> FACKTANGTAIPIGGGSANVYVNLAPVVNVGQNLVVDLSTQIFCHNDYPETITDYVTL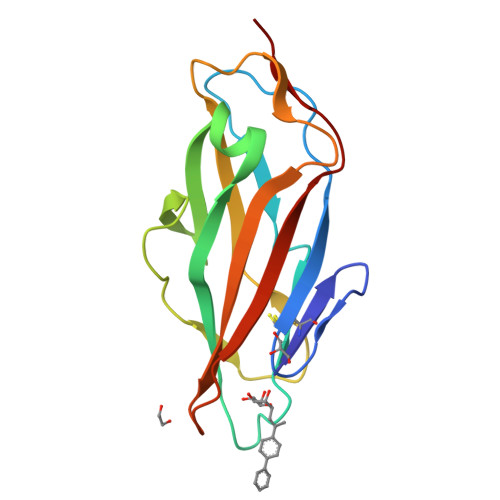QRGSAYGGVLSNFSGTVKYSGSSYPFPTTSETPRVVYNSRTDKPWPVALYLTPVSSAGGVAIKAGSLIAVLILRQTNNYNSDDFQFVWNIYANNDVVVPT> QRRLYDQAKAALAKGNSAPYMASRSALRDYPLEPYLAYDELTHRLKSASNEEVERFLTEHGDLPQIGWLKLRWLRLLADRGDWKTFVNYYDPKLNFTELDCLYGQYQLGHGQK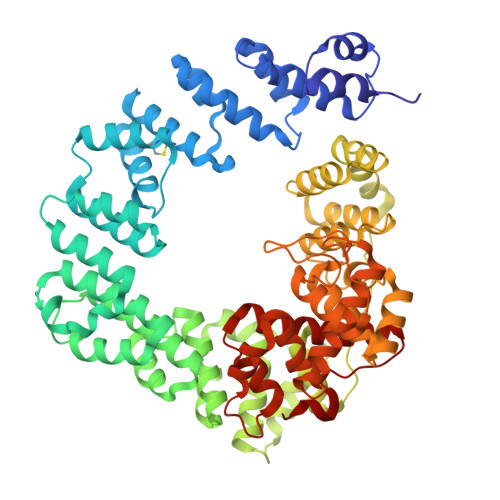AEGYATSERLWLVGKSQPAACDTLFGLWQGEGQLTEEKVWKRLKLAAEARNYSLASHLAQRLPTLGNQGALMVSVAQNPAQLSQTGRFSQRDHATADVVGLGLRRLARQDPEKALSLLDYYSSALPFSSDEKVAIAREIGLSLAKRFDPRALPLMTQYDPGLRDNTVTEWRTRLLLRLGRWDEAYALTRKLPQDLAATSRWRYWQARSLQLAQPNSKEPIALYQKLAGERDFYGFLAADRLSVPYKLGNRPAHIDPRVLQRVRNAASTRRAMEFFNRGEVINARREWYHAARLFDRDELIAQARLAYDMQWYFPAIRSISQAQYWDDLDIRFPMAHRATLVREAKNRGLHSSWIFAITRQESAFMSDARSGVGATGLMQLMPGTAKETSRKFGIPLASTQQLIVPDVNIRLGAAYLSQVHSQFNGNRVLASAAYNAGPGRVRQWLKDTRHLAFDVWIETIPFDETRQYVQNVLSYAVIYGQKLNAPQPIVDWHERYF>MFQPLLDAYVESASIEKMASKSPPPLKIAVANWWGDEEIKEFKNSVLYFILSQRYTITLHQNPNEFSDLVFGNPLGSARKILSYQNAKRVFYTGENESPNFNLFDYAIGFDELDFNDRYLRMPLYYDRLHHKAESVNDTTAPYKLKDNSLYALKKPSHCFKEKHPNLCAVVNDESDPLKRGFASFVASNPNAPIRNAFYDALNSIEPVTGGGSVRNTLGYNVKNKNEFLSQYKFNLCFENTQGYGYVTEKIIDAYFSHTIPIYWGSPSVAKDFNPKSFVNVHDFKNFDEAIDYIKYLHTHKNAYLDMLYENPLNTLDGKAYFYQNLSFKKILAFFKTILENDTIYHDNPFIFCRDLNEPLVTILEHHHH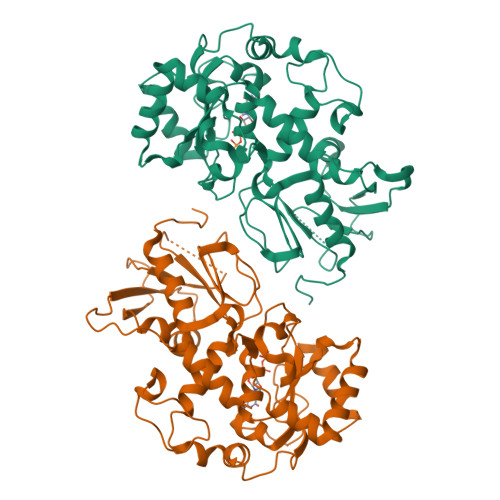HH[3x]> XLYASSN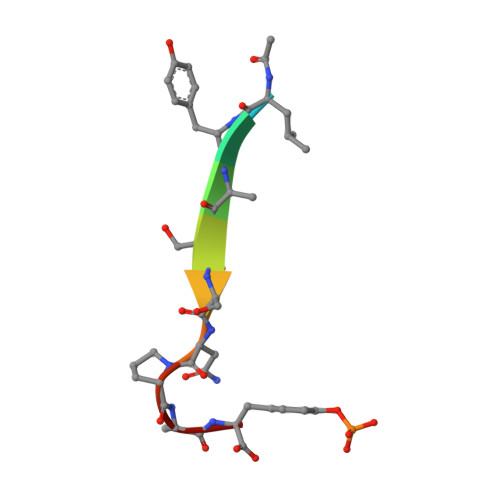PAY> MTSLIDLGRYVERTHHGEDTEPRSKRVKIAKPDLSSFQPGSIIKIRLQDFVTYTLTEFNLSPSLNMIIGPNGSGKSTFVCAVCLGLAGKPEYIGRSKKVEDFIKNGQDVSKIEITLKNSPNVTDIEYIDARDETIKITRIITRSKRRSDYLINDYQVSESVVKTLVAQLNIQLDNLCQFLSQERVEEFARLKSVKLLVETIRSIDASLLDVLDELRELQGNEQSLQKDLDFKKAKIVHLRQESDKLRKSVESLRDFQNK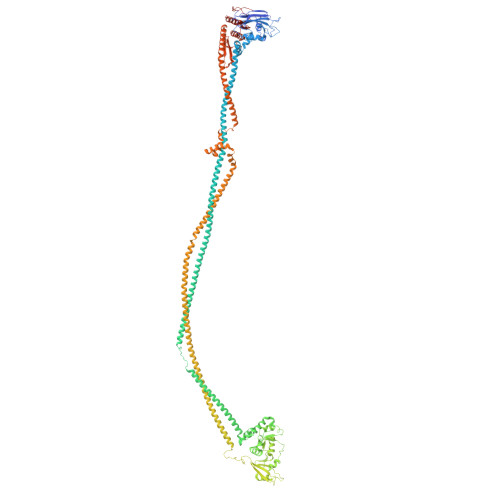KGEIELHSQLLPYVKVKDHKEKLNIYKEEYERAKANLRAILKDKKPFANTKKTLENQVEELTEKCSLKTDEFLKAKEKINEIFEKLNTIRDEVIKKKNQNEYYRGRTKKLQATIISTKEDFLRSQEILAQTHLPEKSVFEDIDIKRKEIINKEGEIRDLISEIDAKANAINHEMRSIQRQAESKTKSLTTTDKIGILNQDQDLKEVRDAVLMVREHPEMKDKILEPPIMTVSAINAQFAAYLAQCVDYNTSKALTVVDSDSYKLFANPILDKFKVNLRELSSADTTPPVPAETVRDLGFEGYLSDFITGDKRVMKMLCQTSKIHTIPVSRRELTPAQIKKLITPRPNGKILFKRIIHGNRLVDIKQSAYGSKQVFPTDVSIKQTNFYQGSIMSNEQKIRIENEIINLKNEYNDRKSTLDALSNQKSGYRHELSELASKNDDINREAHQLNEIRKKYTMRKSTIETLREKLDQLKREARKDVSQKIKDIDDQIQQLLLKQRHLLSKMASSMKSLKNCQKELISTQILQFEAQNMDVSMNDVIGFFNEREADLKSQYEDKKKFVKEMRDTPEFQSWMREIRSYDQDTKEKLNKVAEKYEEEGNFNLSFVQDVLDKLESEIAMVNHDESAVTILDQVTAELRELEHTVPQQSKDLETIKAKLKEDHAVLEPKLDDIVSKISARFARLFNNVGSAGAVRLEKPKDYAEWKIEIMVKFRDNAPLKKLDSHTQSGGERAVSTVLYMIALQEFTSAPFRVVDEINQGMDSRNERIVHKAMVENACAENTSQYFLITPKLLTGLHYHEKMRIHCVMAGSWIPNPSEDPKMIHFGETSNYSFD> MPFPFGKSHKSPADIVKNLKESMAVLEKQDISDKKAEKATEEVSKNLVAMKEILYGTNEKEPQTEAVAQLA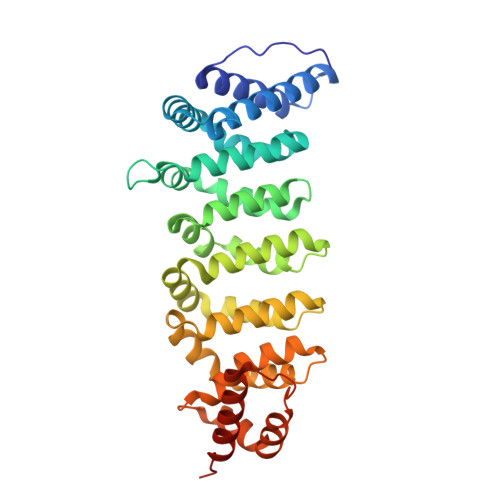QELYNSGLLSTLVADLQLIDFEGKKDVAQIFNNILRRQIGTRTPTVEYICTQQNILFMLLKGYESPEIALNCGIMLRECIRHEPLAKIILWSEQFYDFFRYVEMSTFDIASDAFATFKDLLTRHKLLSAEFLEQHYDRFFSEYEKLLHSENYVTKRQSLKLLGELLLDRHNFTIMTKYISKPENLKLMMNLLRDKSRNIQFEAFHVFKVFVANPNKTQPILDILLKNQAKLIEFLSKFQNDRTEDEQFNDEKTYLVKQIRDLKRPAQQEA>GPHMASAEEKLEKKLELDPNCKEPLQVLPPTVVDQIRLWQLELDRVITYEGSLYSDFETSQEYNLLSKYAQDIGVLLWKDDKKKKFFISKEGNSQVLDFAKRKLKKKQ[2x];>ARARKGALVQCDPS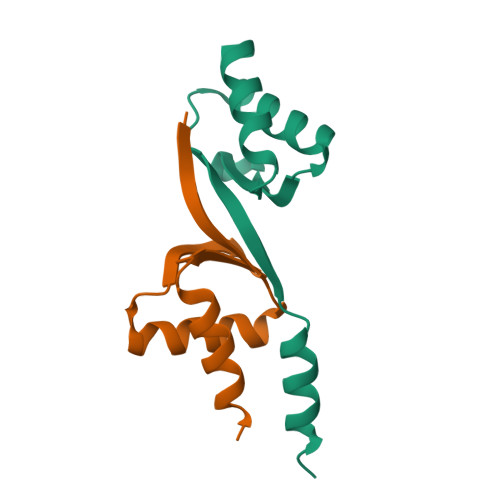IKALILQIDAKMSDIVLEELDDTHLLVNPSKVEFVKHELNRLLSKNIYNPMDEEENQ[2x]>SNAMKILLIGASGTLGSAVKERLEKKAEVITAGRHSGDVTVDITNIDSIKKMYEQVGKVDAIVSATGSATFSP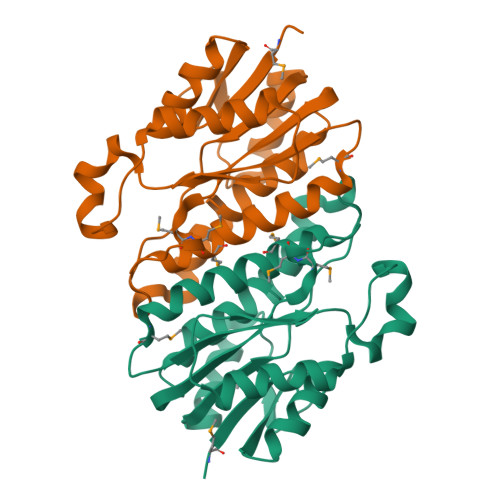LTELTPEKNAVTISSKLGGQINLVLLGIDSLNDKGSFTLTTGIMMEDPIVQGASAAMANGAVTAFAKSAAIEMPRGIRINTVSPNVLEESWDKLEPFFEGFLPVPAAKVARAFEKSVFGAQTGESYQVY[9x]>[2x]MPKKTIFFGAGWFTDRQNKAYKEAMEALKENPTIDLENSYVPLDNQYKGIRVDEHPEYLHDKVWATATYNNNLNGIKTNDIMLGVYIPDEEDVGLGMELG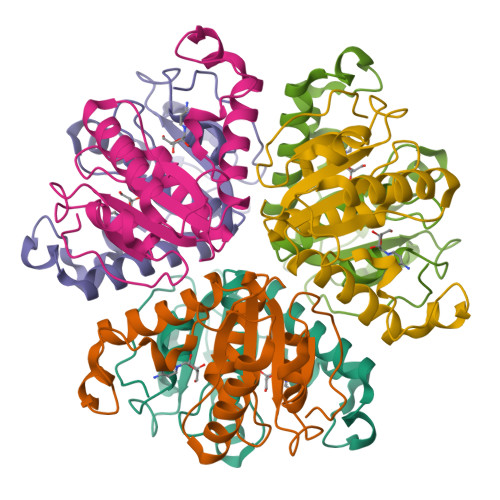YALSQGKYVLLVIPDEDYGKPINLMSWGVSDNVIKMSQLKDFNFNKPRFDFYEGAVY> AVPIAQKSEPHSLSSEALMRRAVSLVTDSTSTFLSQTTYALIEAITEYTKAVYTLTSLYRQYTSLLGKMNSEEEDEVWQVIIGARAEMTSKHQEYLKLETTWMTAVGLSEMAA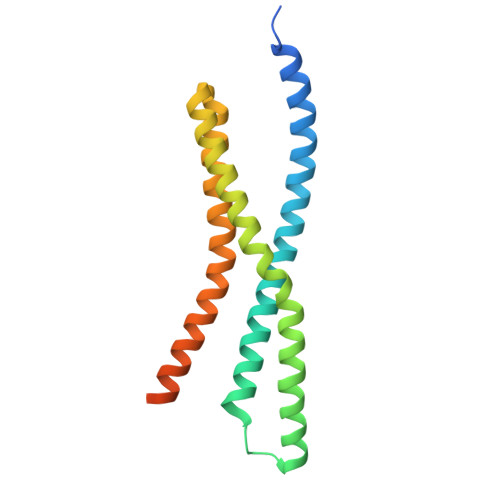EAAYQTGADQASITARNHIQLVKLQVEEVHQLSRKAETKLAEAQIEELRQKTQEEGEERAESEQEAYLRED> MRVALTIAGSDSG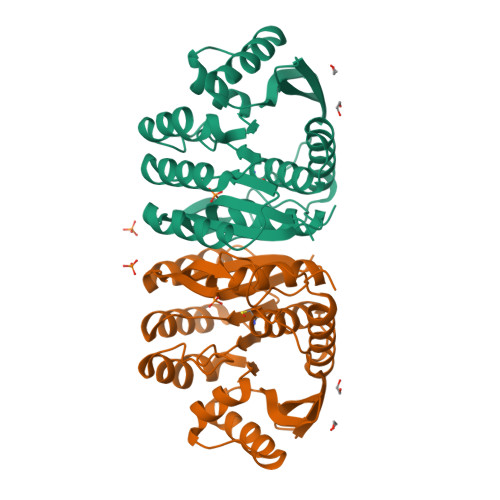GGAGVQADLKTFSRFGVYGMSALTLVTAQNTLGVQRVHLLPPELVYAQIQAVAEDLPIHAAKTGALGNAAIVEAVAEAVRRFGIRPLVVDPVMVAKSGDPLLAPEAVAALKERLFPLATLITPNRLEAEALLGRPIRTLEEAEEAAKALLALGPKAVLLKGGHLEGEEAVDLLATGEGIRRFSAPRVQTRNTHGTGCTLSAAIAALLALGRPLEEAVAEAKAYLTRALETAPSLGHGHGPLNHFA(S)-reticuline | C19 H23 N O4 | 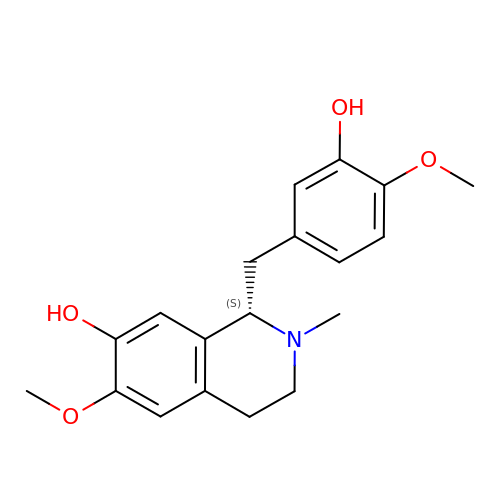BHLYRWXGMIUIHG-HNNXBMFYSA-N> SNAQIDGFVRTLRARPEAGGKVPVFVFHPAGGST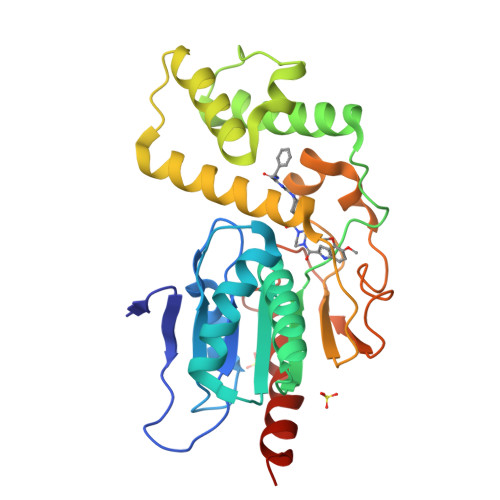VVYEPLLGRLPADTPMYGFERVEGSIEERAQQYVPKLIEMQGDGPYVLVGWSLGGVLAYACAIGLRRLGKDVRFVGLIDAVRAGEEIPQTKEEIRKRWDRYAAFAEKTFNVTIPAIPYEQLEELDDEGQVRFVLDAVSQSGVQIPAGIIEHQRTSYLDNRAIDTAQIQPYDGHVTLYMADRYHDDAIMFEPRYAVRQPDGGWGEYVSDLEVVPIGGEHIQAIDEPIIAKVGEHMSRALGQIEADRTSEVGKQ> SLVFRQLAPNVWQHTSYLDMPGFGAVASNGLIVRDGGRVLVVDTAW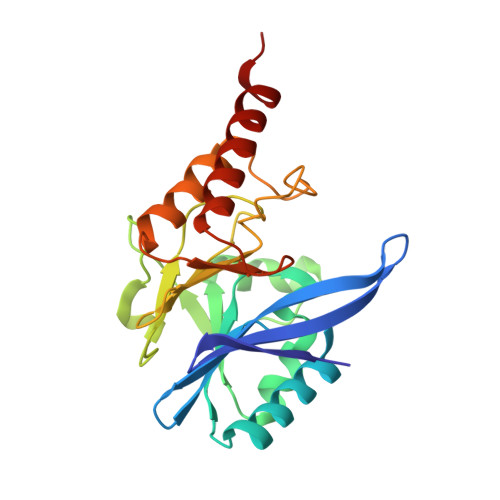TDDQTAQILNWIKQEINLPVALAVVTHAHQDKMGGMDALHAAGIATYANALSNQLAPQEGMVAAQHSLTFAANGWVEPATAPNFGPLKVFYPGPGHTSDNITVGIDGTDIAFGGCLIKDSKAKSLGNLGDADTEHYAASARAFGAAFPKASMIVMSHSAPDSRAAITHTARMADKLRLEHHHHH dibenzothiophene | C12 H8 S | 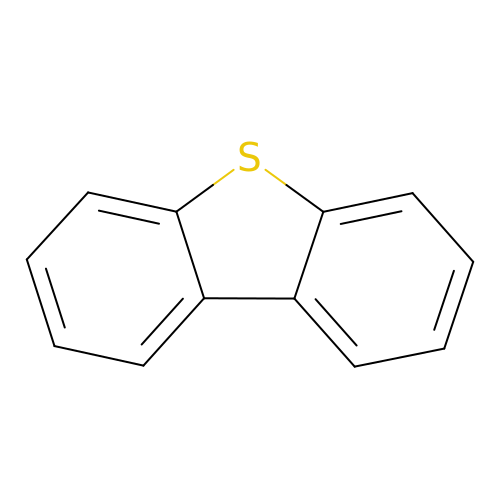IYYZUPMFVPLQIF-UHFFFAOYSA-N> MGLLSLIRGLKKKEGEARILVLGLDNAGKTTILKALSEEDITTITPTQGFNIKSLSRDGFNLKIWDIGGQKSIRPYWRNYFDQTDALI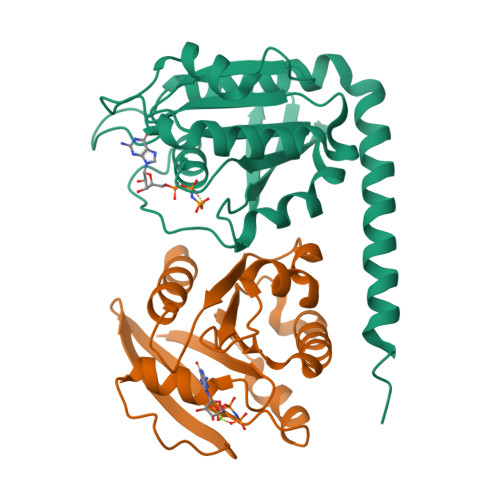YVIDSADSKRLSESEFELTELLQEEKMTGVPLLVFANKQDLVGALAADEIASTLDLTSIRDRPWQIQACSAKQGTGLKEGMEWMMKQVKLEHHHHHH;> GPRKITIALLGLDNAGKTTLLNSIQGEVDRDTTPTFGFNSTTLNEGKYKIEVFDLGGGKNIRGVWKKYLAEVHAIVYVVDAADPGRFEESKMTMAEVLENQFMRDKPICIFANKQDLPTAAPAAEVVKGLGLATCRNSHNVFPCTAKMPAGQDVDHRLRDGLKWLVGTVDREFGRLDPRVQTEAEEVRQEEARKKKEREERLRKQREERLRQQKEEEERAREVEKENELHDGKAPSLLAAGGGVVGAAAAGVNGVMVDEQQEL> GPDSENGVGDAELRERLRQCEETIEQLRAENQELKRKLNILTRPSGILVNDTKLDGPILQILFMNNAISKQYHQEIEEFVSNLVKRFEEQQKNDVEKTSFNLLPQPSSIVLEEDHKVEESCAIKNNKEAFSVVGSVLYFTNFCLDKLGQPLLNENPQLSEGWEIPKYHQVFSHIVSLEGQEIQVKAKRPKPHCFNCGSEEH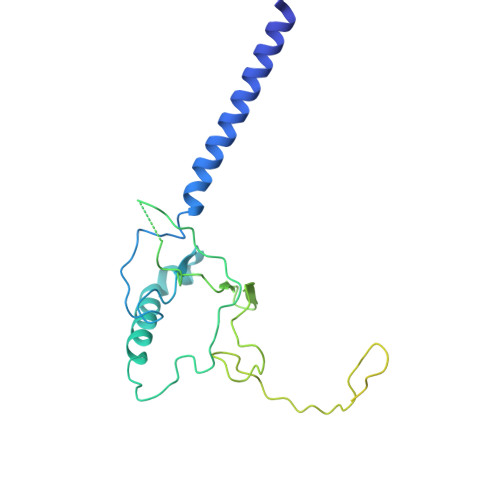QMKDCPMPRNAARISEKRKEYMDACGEANNQNFQQRYHAEEVEERFGRFKPGVISEELQDALGVTDKSLPPFIYRMRQLGYPPGWLKEAELENSGLALYD(5S)-2-amino-5-(2,6-diethylpyridin-4-yl)-3-methyl-5-(3-pyrimidin-5-ylphenyl)-3,5-dihydro-4H-imidazol-4-one 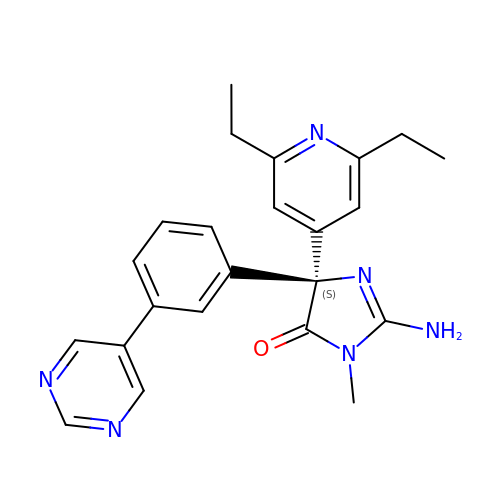| C23 H24 N6 O | QQPRKWVAAAEILV-QHCPKHFHSA-N> DPTEETIKFAAAHYNTEILKSIDNEWRKTQCMPREVAIDVGKEFGVATNTFFKPPCVSVYRCGGCCNSEGLQCMNTSTSYLSKTLFEITVPLSQGPKPVTI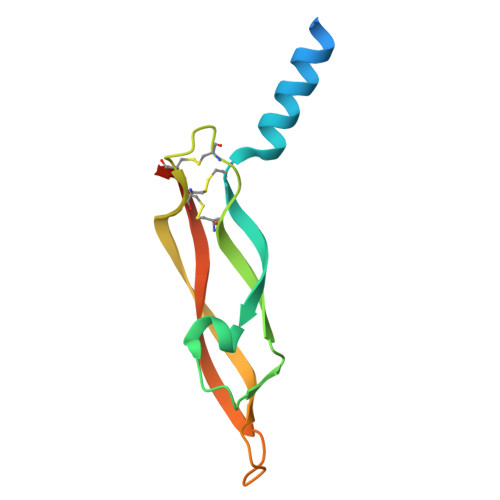SFANHTSCRCMSKLHHHHHH> MSFVKDFKPQALGDTNLFKPIKIGNNELLHRAVIPPLTRMRALHPGNIPNRDWAVEYYTQRAQRPGTMIITEGAFISPQAGGYDNAPGVWSEEQMVEWTKIFNAIHEKKSFVWVQLTVLGWAAFPDNLARDGLRYDSASDNVFMDAEQEAKAKKANNPQHSLTKDEIKQYIKEYVQAAKNSIAAGADGVEIHSANGYLLNQFLDPHSNTRTDEYGGSIENRARFTLEVVDALVEA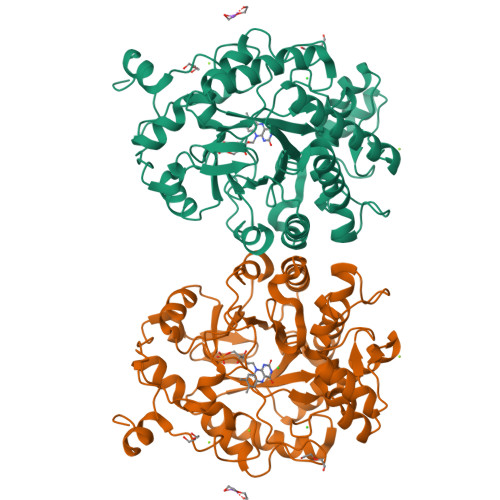IGHEKVGLRLSPYGVFNSMSGGAETGIVAQYAYVAGELEKRAKAGKRLAFVHLVEPRVTNPFLTEGEGEYEGGSNDFVYSIWKGPVIRAGNFALHPEVVREEVKDKRTLIGYGRFFISNPDLVDRLEKGLPLNKYDRDTFYQMSAHGYIDYPTYEEALKLGWDKK> MQVTETVLARAVIKRRSPQLWGAPGAPIIRMRGHHVVWKFQSYDLVVEHTHKRRNSDIRLLHYLGKHCPHPQKSL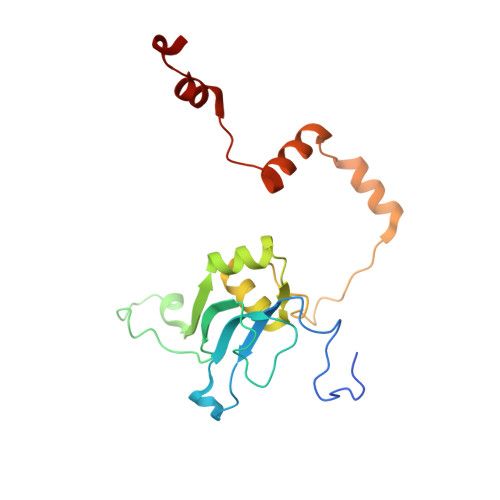WSPDTPVAQDRHLFMLTTVDIDAFKYWFGVKRCRLSMKPWALLAKAGLLPPSLTQNSKIMPKPLFDKESLMRYYLANRKDEDVMAREKYLNYENSMVKTEEERAAERPVAPYL> GSFTMDHYLDIRLRPDPEFPPAQLMCVLFGKLHQALVAQGGDRIGVSFPDLDESRSRLGERLRIHASADDLRALLARPWLEGLRDHLQFGEPAVVPHPTPYRQVSRVQAKSNPERLR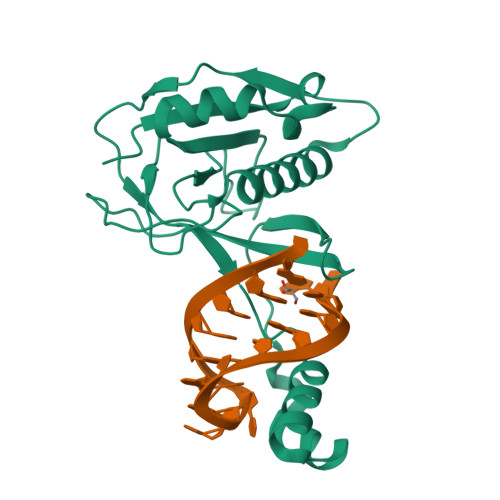RRLMRRHDLSEEEARKRIPDTVARALDLPFVTLRSQSTGQHFRLFIRHGPLQVTAEEGGFTCYGLSKGGFVPWF>GSHMSFRDPTHTPCTAATAAVRAGIDRDTAYGAVTPPIVLSSNFSFDGFGNKRQYDYTRSGNPTRDLLGEALAELEGGAGGVITSTGMGAINLVLNAVLQPGDTLVVPHDAYGGSWRLFNALAKKGH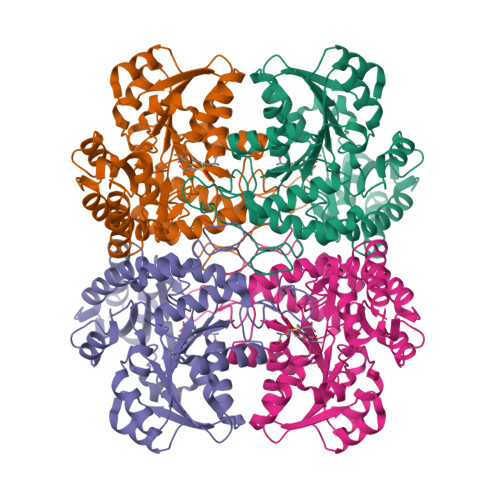FALITADLTVPRSLADALAQSPKLVLIETPSNPLLRITDLRFVIEAAKKVGALTVVDNTFLSPALQKPLDFGADLVLHSTTKYINGHSDVVGGAVVARDAELHQQLVWWANALGLTGSPFDAFLTLRGLRTLDARLRVHQENADAIAELLDGHAMVNQVYFPGLATHPGHALAARQQKGFGAMMSFELEGGEAAVRAFVDGLRYFTLAESLGGVESLIAHPASMTHAAMTAEARAAAGISDGLLRLSIGIESAEDLLIDLRAGLSRAEATLTTTNRKKVDA[4x]FANCM is involved in eukaryotic DNA-damage recognition and activates the Fanconi anemia (FA) pathway through complex formation. MHF is one of the FANCM-associating components and contains a histone-fold DNA-binding domain. The FANCM-associated histone-fold protein (MHF) 1/2 complex (also known as CENP-S/CENP-X) associates with the conserved region of FANCM immediately after the helicase domain to form a FANCM–MHF complex. MHF stabilizes FANCM and promotes its DNA-binding activity.

The purified tripartite complex was crystallized under various conditions and three different crystals were obtained from similar crystallization conditions. Unexpectedly, structure determination revealed that one of the crystals contained the FANCM–MHF complex but that the other two contained the MHF complex without FANCM. The tetrahedral and rod-shaped crystals contained only MHF. Owing to its high resolution, 169 residues and 249 solvent molecules were placed. The root-mean-square displacement (r.m.s.d.) of the heterodimer region was 0.5–0.6 Å. How FANCM dissociates from MHF was further investigated and it was found that the presence of 2-methyl-2,4-pentanediol (MPD) and an oxidative environment may have promoted its release. However, under these conditions MHF retained its complexed form.

> GSEAAGGEQRELLIQRLRAAVHYTTGALAQDVAEDKGVLFSKQTVAAISEITFRQAENFARDLEMFARHAKRSTITSEDVKLLARRSNSLLKYITQKSDELASSNME;> GYEEREGGFRKETVERLLRLHFRDGRTRVNGDALLLMAELLKVFVREAAARAARQAQAEDLEKVDIEHVEKVLPQLLLDFV>[2x]MRALAKLAPEEGLTLVDRP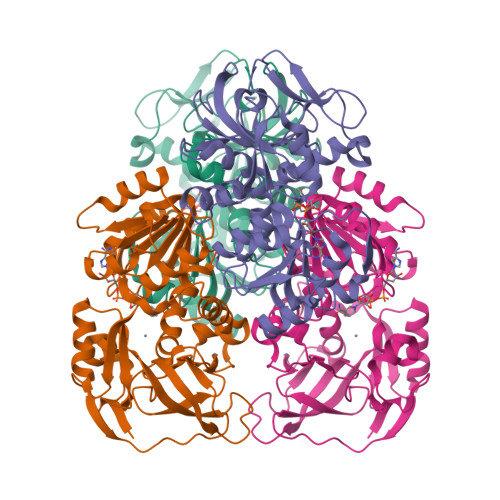VPEPGPGEILVRVEAASICGTDLHIWKWDAWARGRIRPPLVTGHEFSGVVEAVGPGVRRPQVGDHVSLESHIVCHACPACRTGNYHVCLNTQILGVDRDGGFAEYVVVPAENAWVNPKDLPFEVAAILEPFGNAVHTVYAGSGVSGKSVLITGAGPIGLMAAMVVRASGAGPILVSDPNPYRLAFARPYADRLVNPLEEDLLEVVRRVTGSGVEVLLEFSGNEAAIHQGLMALIPGGEARILGIPSDPIRFDLAGELVMRGITAFGIAGRRLWQTWMQGTALVYSGRVDLSPLLTHRLPLSRYREAFGLLASGQAVKVILDPKA> SRLNRESVIDAALELLNETGIDGLTTRKLAQKLGIEQPTLYWHVKNKRALLDALAVEILARHHDYSLPAAGESWQSFLRNNAMSFRRALLRYRDGAKVHLGTRPDEKQYDTVETQLRFMTENGFSLRDGLYAISAVSHFTLGAVLEQQEHTAA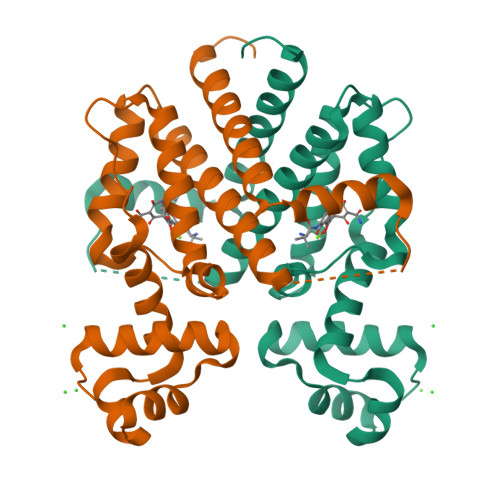LTDRPAAPDENLPPLLREALQIMDSDDGEQAFLHGLESLIRGFEVQLTALLQIV> MRIILLGAPGAGKGTQAQFIMEKYGIPQISTGDMLRAAVKSGSELGKQAKDIMDAGKLVTDELVIALVRERICQEDSRNGFLLDGFPRTIPQADAMKEAGINVDYVLEFDVPDELIVDRIVGRRVHA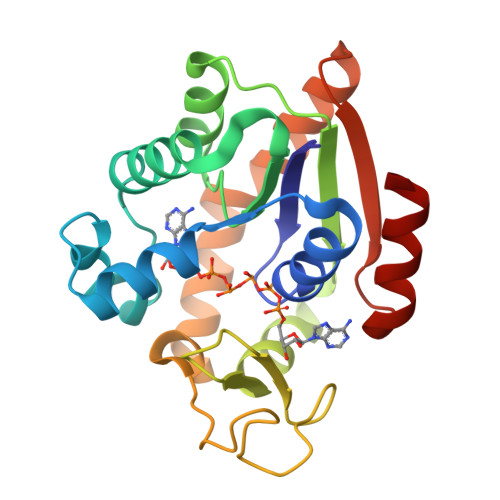PSGRVYHVKFNPPKVEGKDDVTGEELTTRKDDQEETVRKRLVEYHQMTAPLIGYYSKEAEAGNTKYAKVDGTKPVCEVRADLEKILG>ICSGPQNLAQELKAIGDQLQELQKKLIQGPNISQPRPLLTIETPRHLGEQLNARRKELGIDLYTLELQTGISTSTLKRLFKDPEQV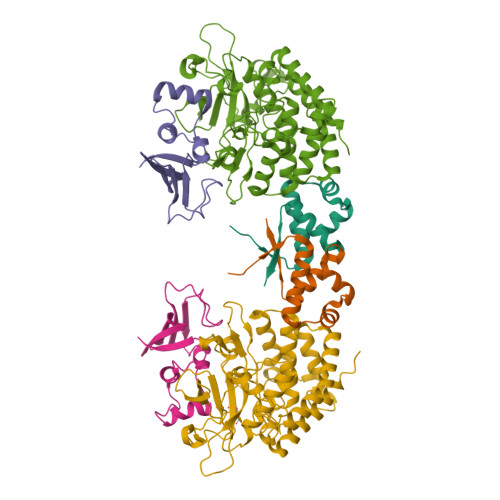KFGSVFAVANVLGVKLCIGE[2x];>HRRVKVLLYGQVVGELSQNDSGFLFQYAHDYHGPAISISLPVAQRQFPSETLHPYFASLAPEGWLRQRYSQIQHRDENDLLGMLIDNGKNLLGAIQILPWEE[2x];>[2x]ANCRILLTPLNERDEQRGYSTQGLKRLSGTAKLNPRLGFTRTQFVQELPRQQKGMSIAGYQPKLQLVLDEGEFRVVDHQGNFILKPSPADFPGLAENEHATMTLMSRLGFDVPVHGLLSFAPQSEEELEYAFVIRRYDRDNKGLPVHQEQLDGAMQITDKYGKTGNDNEQYVSYETLARFLVAHVNDNIAFKIDLFRRIVYAWLLGNNDMHLRNFGLVYSDGLTPALAPVYDFVSVAPYPEYFYSNYLALPLLTREEGGRELAPGFHSDYGEYIGQDFLLLGESMGLAPRLLEKLFQDIRKENAIVMETYEQSFMTQDHIQAVLQCYRHRLGLLHHHHHH> MAVPETRPNHTIYINNLNEKIKKDELKKSLHAIFSRFGQILDILVSRSLKMRGQAFVIFKEVSSATNALRSMQGFPFYDKPMRIQYAKTDSDIIAKMKGT

The catalytic activity of the HDV ribozyme is essential for viral replication and viral particle assembly inside the host cells. In addition, residue C75 (C76 in the antigenomic ribozyme) is essential for the cleavage reaction, and mutating C75 to any other base, especially uracil or guanine, inhibits the reaction. In this study, we have used these new techniques to correct and improve the cleaved and the cis-acting C75U-inhibited structures of the HDV ribozyme, which were originally solved over a decade ago.

To prevent catalysis in the crystal structure of the HDV ribozyme, the catalytic residue C75 was mutated to a uracil. The C75U-inhibited structure 1VC7 was solved at 2.45Å resolution and has R = 23.91% and Rfree = 26.40%, as calculated by PHENIX with anisotropic B factors from the original TLS refinement. After several cycles of automated rebuilding using tools described before, evaluation of their output, and sporadic manual rebuilding, alternated with rounds of refinement in PHENIX, the structure was significantly improved. All geometry and ribose pucker outliers were corrected, including 10 ribose puckers that were misfit as either C3′-endo or O4′-endo and now corrected to C2′-endo. ERRASER fixed the errors in the RNA backbone and, despite our exerting no direct control over the arrangement of the G25:U20 base pair, flipped the G25 residue, replacing the original Hoogsteen base pair by a reverse GU wobble base pair with two hydrogen bonds. The reverse GU wobble base pair positions the O6 atom on G25 to interact with the active site metal ion in the C75U-inhibited structure, but no metal ion is bound in the cleaved structure. The final model of the two upstream nucleotides, although not fit or refined with alternate conformations, shows electron density accounting for perhaps 80% of full occupancy, so the C75U mutation indeed succeeded in producing an uncleaved structure. The backbone suite between U -1 and G1 is now fit very satisfactorily, but the U -1 O2′ is still 9Å from the metal, and the position and orientation of the scissile bond is even less appropriate for catalysis than in 1VC7. In addition, the coordination of Sr2+ by the O4 atom of U75 is an artefact of the C75U mutation, as an exocyclic amino group replaces the O4 atom in the wild-type ribozyme. The rebuilt structure was refined with two TLS groups, one for the RNA chain and one for the protein chain, and has R = 19.80% and Rfree = 25.13%, an improvement of 4.11 and 1.27%, respectively.>MVAVP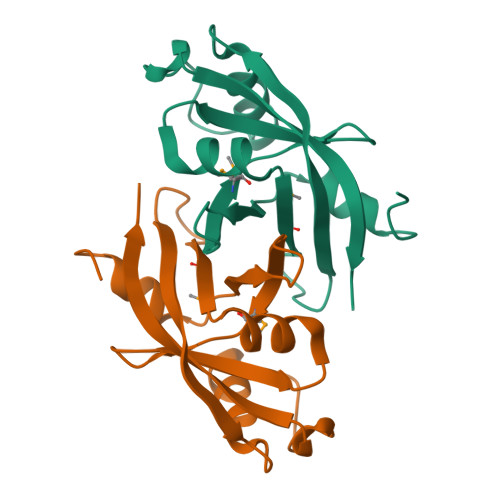EGYESLLERPLYGHLATVRPDGTPQVNAMWFAWDGEVLRFTHTTKRQKYRNIKANPAVAMSVIDPDNPYRYLEVRGLVEDIVPDPTGAFYLKLNDRYDGPLTEPPADKADRVIIVVRPTAFSKQVA[2x]> MADLRKAARGRECQVRIPGVCNGNPETSVLAHIRLTGLCGTGTKPPDLIATIACSACHDEIDRRTHFVDAGYAKECALEGMARTQVIWL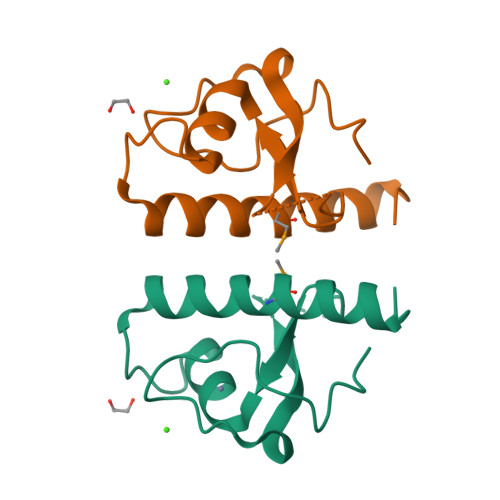KEGVIKA>[2x]GHMKASSRRTISQNKRRYRKDGFDLDLTYVTDHVIAMSFPSSGRQSLFRNPIGEVSRFFKTKHPDKFRIYNLCSERGYDETKFDNHVYRVMIDDHNVPTLVDLLKFIDDAKVWMTSDPDHVIAIHSKGGKGRTGTLVSSWLLEDGKFDTAKEALEYFGSRRTDFEVGDVFQGVETASQIRYVGYFEKIKKNYGGQLPPMKKLKVTGVTITAIQGVGRGNGSDLSMQIVSERQEVLLCKFAEGYNCALQYD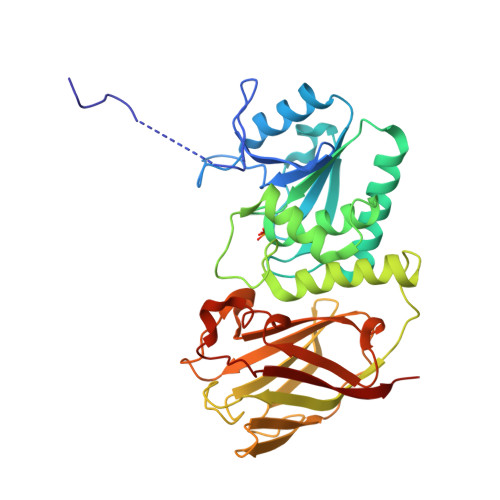ATDDCVTCEVKNCPVLAGDIKVRFMSTSKSLPRGYDNCPFYFWFNTSLVEGDHVTLKREEIDNPHKKKTWKIYRDNFTVKLTFSDAEDI> SGLVPRGSHMRLRPLGIEGVWEITPEQRADPRGVFLDWYHVDRFAEAIGRPLRLAQANLSVSVRGVVRGIHFVDVPPGQAKYVTCVRGAVFDVVVDLRVGSPTYGCWEGTRLDDVSRRAVYLSEGIGHGFC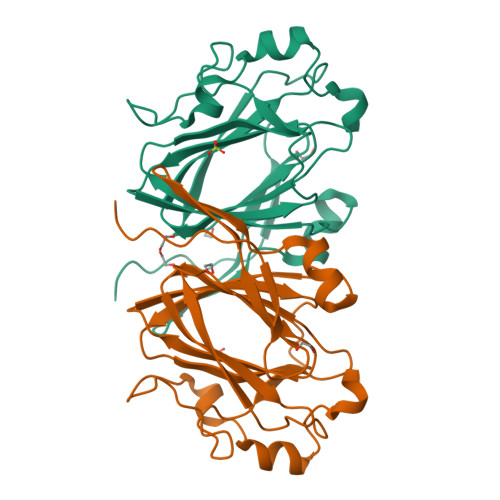AISDEATLCYLSSGTYDPATEHGVHPLDPELAIDWPTGTPLLSPRDQDALLLAEARDAGLLPTYATCQAVTVPSPAPGSVGDPGP> GSSLGTVDAPNFIVGNPWDDKLIFKLLSGLSKPVSSYPNTFEWQCKLPAIKPKTEFQLGSKLVYVHHLLGEGAFAQVYEATQGDLNDAKNKQKFVLKVQKPANPWEFYIGTQLMERLKPSMQHMFMKFYSAHLFQNGSVLVGELYSYGTLLNAINLYKNTPEKVMPQGLVISFAMRMLYMIEQVHDCEIIHGDIKPDNFILGNGFLEQDDEDDLSAGLALIDLGQSIDMKLFPKGTIFTAKCETSGFQCVEMLSNKPWNYQIDYFGVAATVYCMLFGTYMKVKNEGGECKPEGLFRRLPHLDMW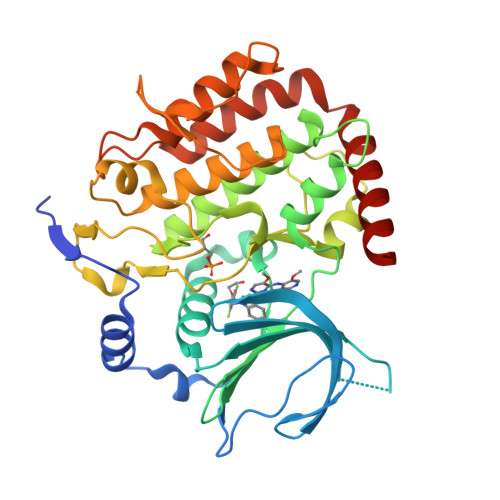NEFFHVMLNIPDCHHLPSLDLLRQKLKKVFQQHYTNKIRALRNRLIVLLLECKRSRK> MRYCRPSRPLVLARASSVLSSSRTFHSQHRTPIIPQVHVHDEPTAQRIHVGYYLHRHPVVKHSPHPLE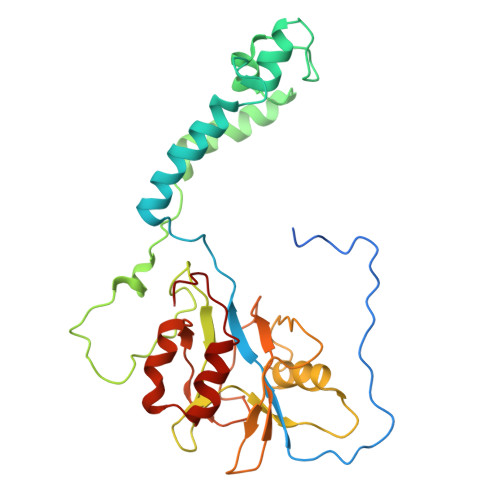TEMGYLLEREQQRYSRHESAESATAFFASRGQTIDILGRTDPNQIKGNFFGLELYQDAMKVVMQRYTPEKRLTSADLWQPNALGDAPPPRHTLHRKLDDFLYLIVQEGATGKWTIPHTARKDDESLRMTADRAISSQNSEGLDCYVWSNAPQATVFLKDDNTRLFIYAATYLAGRPQFASFEPKPKDHAWVTRHELLQYSDTFKSAELLKALLDISADGTFEA>[4x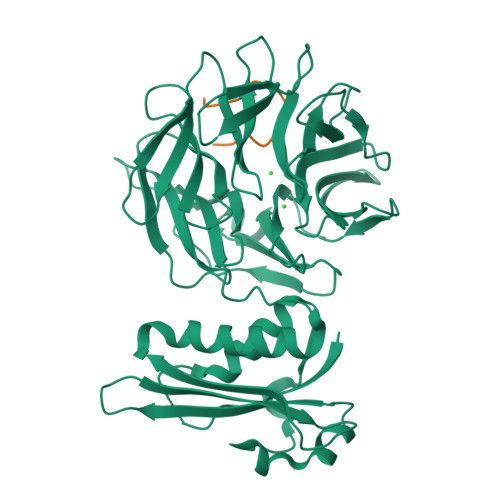]MMKQALRVAFGFLILWASVLHAEVRIVIDSGVDSGRPIGVVPFQWAGPGAAPEDIGGIVAADLRNSGKFNPLDRARLPQQPGSAQEVQPAAWSALGIDAVVVGQVTPNPDGSYNVAYQLVDTGGAPGTVLAQNSYKVNKQWLRYAGHTASDEVFEKLTGIKGAFRTRIAYVVQTNGGQFPYELRVSDYDGYNQFVVHRSPQPLMSPAWSPDGSKLAYVTFESGRSALVIQTLANGAVRQVASFPRHNGAPAFSPDGSKLAFALSKTGSLNLYVMDLASGQIRQVTDGRSNNTEPTWFPDSQNLAFTSDQAGRPQVYKVNINGGAPQRITWEGSQNQDADVSSDGKFMVMVSSNGGQQHIAKQDLATGGVQVLSSTFLDETPSLAPNGTMVIYSSSQGMGSVLNLVSTDGRFKARLPATDGQVKFPAWSPYLLEHHHHHH;>[4x]GASDGSGWSSENNPWG2,5-BIS-[4-[CYCLOPENTA-1,3-DIEN-5-YLAMINO-1-AMINOMETHYL]-PHEN-1-YL]FURAN 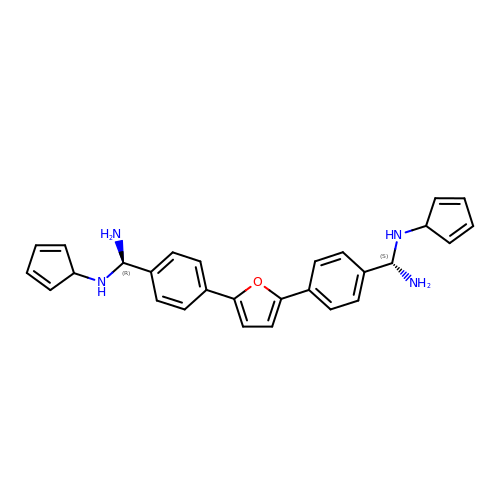| C28 H28 N4 O | IKWANHYVTLMFON-HNRBIFIRSA-N>KVTMNDFDYLKLLGKGTFGKVILVREKATGRYYAMKILRKEVIIAKDEVAHTVTESRVLQNTRHPFLTALKYAFQTHDRLCFVMEYANGGELFFHLSRERVFTEERARFYGAEIVSALEYLHSRDVVYRDIKLENLMLDKDGHIKITDFGLCKEGISDGATMKTFCGTPEYLAPEVLEDNDYGRAVDWWGLGVVMYEMMCGRLPFYNQDHERLFELILMEEIRFPRTLSPEAKSLLAGLLKKDPKQRLGGGPSDAKEVMEHRFFLSINWQDVVQKKLLPPFKPQVTSEVDTRYFDDEFTAQSITITPPDRYDSLGLLELDQRTHFPQFDYSASIR[2x];>[2x]GR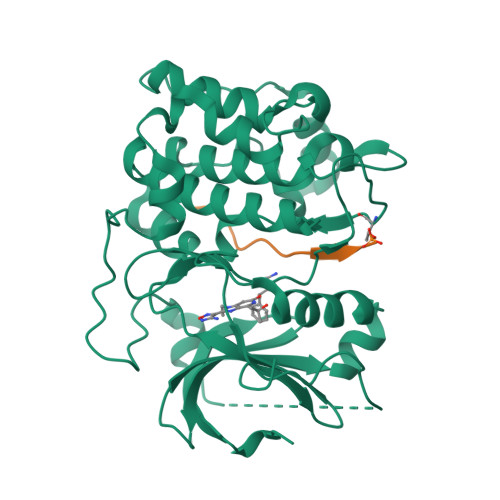PRTTSFAE>MHHHHHHMRMIQKFEGKKPEIHETAFVHPRATIIGDVEIGPKTSVWPGAVIRADIEKITIGKNTCIKDNAVIHPADVYHEEEIEYVPVKIGDNNIIGHRALIHGAKINDESIVGAGSIVFNKAEVKTN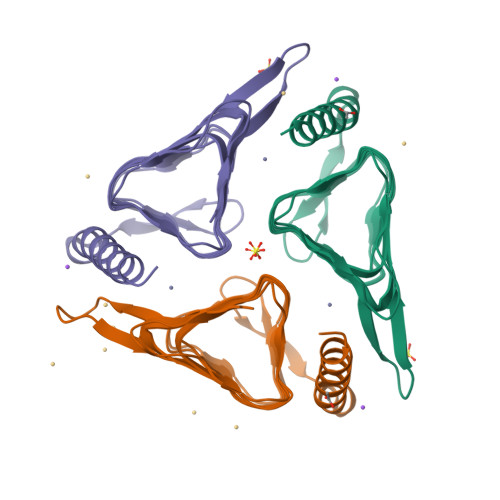SMVGMGAVVLEKQEVPNGKIVVGIPARVLRELEEREIKQIKKQADTHAELAEHYSREIEEP[5x]>MASKPTLKEVVIVSATRTPIGSFLGSLSLLPATKLGSIAIQGAIEKAGIPKEEVKEAYMGNVLQGGEGQAPTRQAVLGAGLPISTPCTTINKVCASGMKAIMMASQSLMCGHQDVMVAGGMESMSNVPYVMNRGSTPYGGVKLEDLIVKDGLTDVYNKIHMGSCAENTAKKLNIARNEQDAYAINSYTRSKAAWEAGKFGNEVIPVTVTVKGQPDVVVKEDEEYKRVDFSKVPKLKTVFQKENGTVTAANASTLNDGAAALVLMTADAAKRLNVTPLARIVAFADAAVEPIDFPIAPVYAASMVLKDVGLKKEDIAMWEVNEAFSLVVLANIKMLE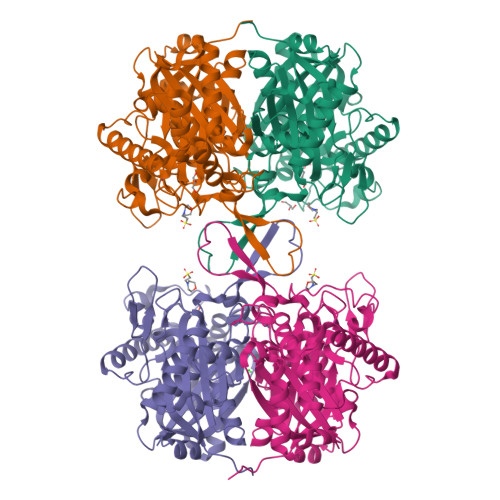IDPQKVNINGGAVSLGHPIGMSGARIVGHLTHALKQGEYGLASICNGGGGASAMLIQKL[4x]>[2x]GPMDPSSLGTVDAPNFIVGNPWDDKLIFKLLSGLSKPVSSYPNTFEWQCKLPAIKPKTEFQLGSKLVYVHHLLGEGAFAQVYEATQGDLNDAKNKQKFVLKVQKPANPWEFYIGTQLMERLKPSMQHMFMKFYSAHLFQNGSVLVGELYSYGTLLNAINLYKNTPEKVMPQGLVI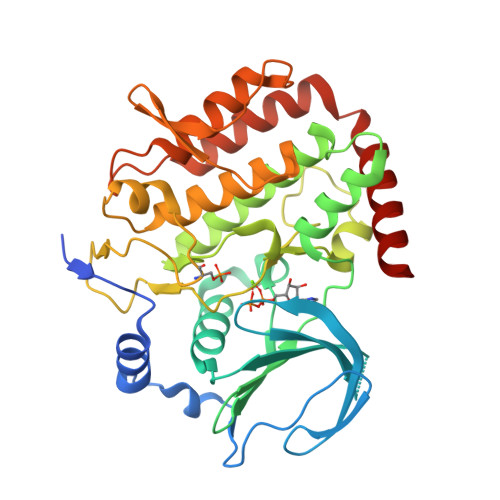SFAMRMLYMIEQVHDCEIIHGDIKPDNFILGNGFLEQDDEDDLSAGLALIDLGQSIDMKLFPKGTIFTAKCETSGFQCVEMLSNKPWNYQIDYFGVAATVYCMLFGTYMKVKNEGGECKPEGLFRRLPHLDMWNEFFHVMLNIPDCHHLPSLDLLRQKLKKVFQQHYTNKIRALRNRLIVLLLECKRSRK>SNAMKKTATPKLRLLLSNDDGVYAKGLAILAKTLADLGEVDVVAPDRNRSGASNSLTLNA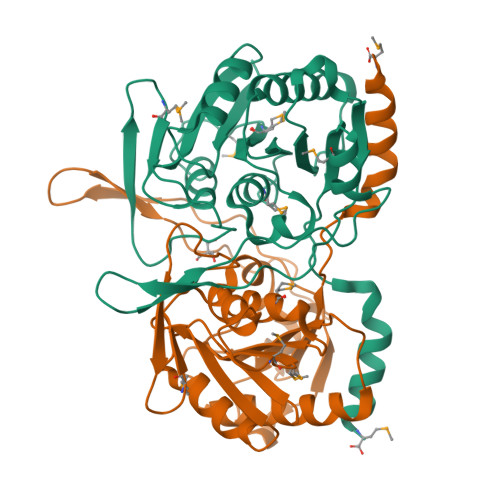PLHIKNLENGMISVEGTPTDCVHLAITGVLPEMPDMVVAGINAGPNLGDDVWYSGTVAAAMEGRFLGLPALAVSLGGELFRYYETAAKVVYQLIQRIEKDPLPPSTILNINVPDLPYEELKGFEVTRLGTRHRAEPTIRQIDPRGHPIYWVGAAGPEQDSGPGTDFFAMNHHCVSITPLRVDLTHYEAFDQLASWVKRLEM[2x]> GSHMDYLVTEEEINLTRGPSGLGFNIVGGTDQQYVSNDSGIYVSRIKENGAAALDGRLQEGDKILSVNGQDLKNLLHQDAVDLFRNAGYAVSLRVQHRLQVQGSAYGSVKAYTNFDAERDALNIETAIKTKGVDEVTIVNILTNRSNEQRQDIAFAYQRRTKKELASALKSALSGHLETVILGLLKTPAQYDASELKASMKGLGTDEDSLIEIICSRTNQELQEINRVYKEMYKTDLEKDIISDTSGDFRKLMVALAKGRRAEDGSVIDYELIDQDARDLYDAGVKRKGTDVPKWISIMTERSVPHLQKVFDRYKSYSPYDMLESIRKEVKGDLENAFLNLVQCIQNKPLYFADRLYDSMKGKGTRDKVLIRIMVSRSEVDMLKIRSEFKRKYGKSLYYYIQQDTKGDYQKALLYLCGGDD;> TDDSRRVRKLPSTTL

The human proteome comprises 266 human PDZ (PSD95/DLG1/ZO1) domains 16 and about 4000 putative PBMs, defining a network of one million potential interactions. PBMs are mostly (though not exclusively) C-terminal, with their COO- implicated in binding, and are classified based on position −2, being respectively Ser/Thr, hydrophobic or acidic in classes 1, 2, and 3 17,18. PDZ-PBM interactions are rather transient and promiscuous. Viral proteins bearing functional PBMs are found notably in HPV and HTLV oncoviruses as well as in HBV, WNV and coronaviruses including MERS or SARS-CoV213,15,23–26.

In another example, the profile and the logo of SYNJ2BP indicate that this PDZ-domain is highly promiscuous, with however a mild preference for E-T-x-V-COO- motifs and a moderate bias for basic residues at upstream (−4 and −5) positions. RPS6KA1 PBM does not fully match SYNJ2BP’s logo and thus binds only weakly to SYNJ2BP (pKd = 3.82). Upon phosphorylation at p-3, RPS6KA1 gains a negative charge at this position, thereby getting closer to SYNJ2BP’s logo. Accordingly, the p-3 phosphorylated variant RPS6KA1 gains affinity to SYNJ2BP (pKd = 4.48; ΔpKd = 0.66), as previously published. The structure of p-3 phosphorylated RPS6KA1 bound to SYNJ2BP explains this enhanced binding by revealing a network of specific phosphoryl-PDZ contacts. The p-3 phosphorylated RPS6KA1 PBM matches better to SYNJ2BP logo, with acidic phospho-Ser at p-3 contacting two residues of SYNJ2BP β2 and β3 strands in the complex. Nonetheless, p-3 phosphorylated RPS6KA1 binds only mildly to SYNJ2BP as compared to SYNJ2BP’s strongest binder in our interactome, the oncoviral PBM of HTLV1 Tax1 (pKd = 6.04). Yet Tax1 matches better than phosphorylated RPS6KA1 to SYNJ2BP’s logo thanks to a basic p-4 Arg and a p0 Val (Pro and Leu in RPS6KA1, respectively). Accordingly, in the crystal structures, p-4 Arg of Tax1 establishes favorable H-bonds with a Gln from the α2 helix of SYNJ2BP PDZ, and the Val-bound state of SYNJ2BP PDZ is more compact than its Leu-bound state, due to displacement of the carboxylate-binding GLGF loop likely driven by the larger side-chain of Leu. The carboxylate-binding loop of SYNJ2BP is shifted in the phosphorylated RPS6KA1-bound complex, most likely related to unfavorable Val → Leu substitution at p0 of RPS6KA1 PBM.>MIFTNAILVISALLPATVLSLQHTEDSLFPARCWPDPCAGITFQNDTYVCGDPRLGPVVLPQKFPLNNELRTYARFGALCPAEFLDKWATDVAPNGTYIYPPANGFALDTEEQPILGNATLPVGMKLDRFGSEYGTFLAPLGAPYIERSLPPSNLNTFDGMYPYNYHVYQVTKEFVVGLGPIAPWFEQPGMGTQFVTYTNVLGLIDDGYLRRLDESEYDEKVEYSNPYTPGPNQDVLFQG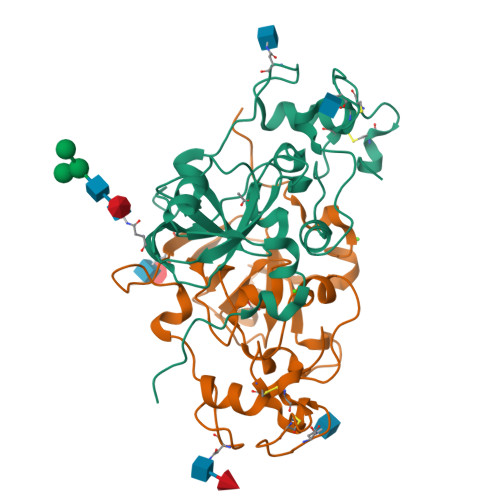PGHHHHHH[2x]The recently discovered arginine rhamnosylation activates the polyproline-specific bacterial translation elongation factor EF-P. EF-P is rhamnosylated on arginine 32 by the glycosyltransferase EarP. Rhamnosylation is mediated by the recently discovered inverting glycosyltransferase EarP, which utilizes dTDP-beta-l-rhamnose (TDP-Rha) as donor substrate, resulting in α-rhamnosyl-arginine on the acceptor EF-P. Unlike with the common and relatively well understood glycosylation of asparagine, sugar modifications on the guanidino group of arginine appear to be rare, and almost nothing is known about the molecular mechanism. The enzyme is composed of two opposing domains with Rossmann folds, thus constituting a B pattern-type glycosyltransferase (GT-B). While dTDP-β-l-rhamnose is located within a highly conserved pocket of the C-domain, EarP recognizes the KOW-like N-domain of EF-P. Based on our data, we propose a structural model for arginine glycosylation by EarP.

We were able to subsequently confirm the GT-B fold by having solved the crystal structure of EarPPpu at 2.3-Å resolution (Data Set S2). Indeed, the EarPPpu C-domain includes residues 184 to 361 and follows the Rossmann fold topology, with six β-strands (β8 to β13) and seven α-helices (α8 to α14). On the other hand, the N-domain (aa 1 to 153 and 362 to 377) could only be built in part. Yet, the structure has a higher-than-usual R-free (35.1%) value at this resolution, which cannot be explained by a simple absence of disordered regions. This is likely due to the N-domain adopting different conformations in different unit cells, causing crystal disorder. Similarly, TDP-Rha in the EarPPpu crystal structure is located in a binding pocket that is composed of residues located in the C-domain. F191EarP, F252EarP, and F258EarP side chains form an aromatic cage that stacks against the base of the nucleotide moiety of TDP-Rha. The sugar ring of the nucleotide is then specifically recognized by a hydrogen bond between the hydroxyl group on C3′ of the sugar and the side chain of Q255EarP. The diphosphate is recognized by hydrogen bonds formed with the side chain guanidine of R271EarP, the Y193EarP side chain hydroxyl, and backbone amides of E273EarP and D274EarP. The binding pocket is closed by the bulky side chain of Y193EarP, which may sterically ensure proper positioning of the rhamnose sugar. The rhamnose sugar itself does not seem to make any contact with the protein and is solvent exposed.

> MGSSHHHHHHSQDPKATWDIFCSVVDNYGDIGVTWRLARQLVAEHGLAVRLWVDDLNAFTPMCPGADATAAQQWQHGVDVRHWPAAWLPVAPADVVIGAFACQLPAAYVEAMRARPQPPLWLNLEYLSAEDWVEGCHGLPSPQPNGLRKVFFFPGFTDKTGGLLREGSLLARRDGFQQSAEARRAFLQGLGVDLVPGALLISLFAYENPQLGNWLDALATADQPCHLLVPQGRVVAGLSQWLGEGPLHVGDVRTRGALTVQVLPFVSQDDFDRLLWSCDFNAVRGEDSFVRAQWAGQPMLWHIYVQDENAHWEKLEAFLAHYRCGLSDDADAALLGLWRAWNMDFDMGQAWRAARQHWPELQQHARLWGARQAAQPDLATALVHFYRNSL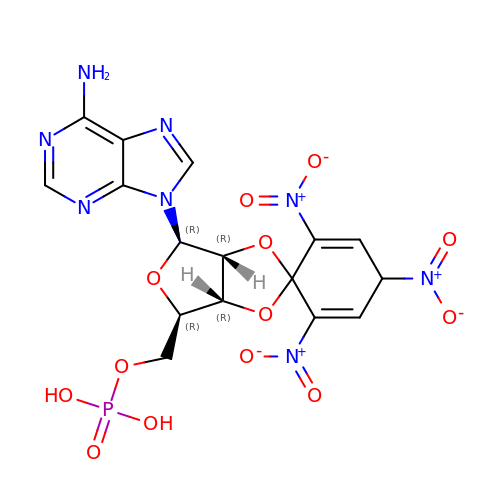2',3'-O-[(1r)-2,4,6-trinitrocyclohexa-2,5-diene-1,1-diyl]adenosine 5'-(dihydrogen phosphate) | C16 H15 N8 O13 P | OHPXFACYTRBVRA-DLHKNTDHSA-N> GPLSFSLGLQDFDLLRVIGRGSYAKVLLVRLKKTDRIYAMKVVKKELVNDDEDIDWVQTEKHVFEQASNHPFLVGLHSCFQTESRLFFVIEYVNGGDLMFHMQRQRKLPEEHARFYSAEISLALNYLHERGIIYRDLKLDNVLLDSEGHIKLTDYGMCKEGLRPGDTTSTFCGTPNYIAPEILRGEDYGFSVDWWALGVLMFEMMAGRSPFDIVGSSDNPDQNTEDYLFQVILEKQIRIPRSLSVKAASVLKSFLNKDPKERLGCHPQTGFADIQGHPFFRNVDWDMMEQKQVVPPFKPNISGEFGLDNFDSQFTNEPVQLTPDDDDIVRKIDQSEFEGFEYINPLLMSAEECV;> LAFQREGFGRQSMSEKRTKQ

Atypical protein kinase C (aPKC) is a key apical-basal polarity determinant and Par complex component. The atypical protein kinase C (aPKC in Drosophila or PKCι/PKCζ isozymes in mammals), its binding partner Par6, and the small guanosine triphosphatase Cdc42 are three essential determinants of apical membrane identity in both Drosophila and mammals (Fletcher et al., 2012, Harris and Tepass, 2008, Hutterer et al., 2004, Izumi et al., 1998, Joberty et al., 2000, Lin et al., 2000, Wodarz et al., 2000). aPKC isoforms PKCι and PKCζ have regulatory regions distinct from those of other PKC isozymes, but share a conserved catalytic protein kinase domain. Like many protein kinases, activation of aPKC requires activation-loop phosphorylation and an αC-helix conformation compatible with Lys-Glu salt-bridge formation to bind ATP and serve to align residues within the R spine (Kornev et al., 2008).

To understand how Par3CR3 could inhibit PKCιKD-2P, we determined the 2.0-Å crystal structure of a longer Par3 peptide (residues 816–841) bound to PKCιKD-2P and Mg-AMPPNP (adenylyl imidodiphosphate). It engages PKCιKD-2P by adopting a “staple”-shaped conformation with two arms that flank the S827Par3 phospho-acceptor site. Each arm binds in close proximity to opposite ends of the nucleotide, suggesting that recognition of aPKC is driven by nucleotide occupancy. Par3CR3 contacts extend from a pocket beneath the ribose-binding pocket of PKCι (site 1), across the G helix (site 2) through to the activation loop, αB and αC helices of the PKCιKD-2P N lobe (site 3). The amino-terminal part of Par3CR3 binds to site 1 (PKCιKD-2P kinase C lobe) through an F-X-R motif at positions −9 (F−9) and −7 (R−7) defined relative to the phospho-acceptor (P site) at serine 0 (equivalent to S827 of human Par3). The phospho-acceptor serine-0 hydroxyl hydrogen bonds to side chains of D378PKCι, K380PKCι, and T416PKCι, preventing a catalytically competent orientation for nucleophilic attack on the ATP γ-phosphate. We define this portion of Par3CR3 as the “inhibitory arm,” as it directly perturbs an active PKCιKD-2P N-lobe conformation (discussed later). Crucially, the R+5 side chain is buried within a hydrophobic pocket beneath the regulatory αC helix. The pocket is lined by side chains from Y265PKCι on the glycine loop and W298PKCι of the αC helix, each making π-stacking interactions with the guanidino group of R+5. Overall, the structure reveals that the Par3CR3 clamp involves an “inhibitory arm” and an “anchoring arm,” which together recognize and inhibit a nucleotide-bound PKCιKD-2P conformer.Cys-loop receptors are allosterically regulated pentameric ligand-gated ion channels (pLGICs). In this work, we studied orphan receptor Alpo4 from an extreme thermophile worm Alvinella pompejana. Each Alpo4 subunit is composed of a β-sandwich extracellular domain (ECD) and a transmembrane domain (TMD) made of four trans-membrane α-helices M1-M4. In conclusion, Alpo4 has a pore structure consistent with a cation-selective channel, but with an unusually tight constriction at the 16’M position, the role of which remains unclear.

Given that Alpo4 shares a structural resemblance to the α4β2 nAChR and the 5-HT3R, we investigated whether acetylcholine or serotonin binds into the ligand-binding site. To this end, structures of Alpo4 purified in the absence of CHAPS and with an added, 1 mM acetylcholine or 1 mM serotonin were solved to a resolution of 3.9 Å and 6.2 Å, respectively (Figure 1—figure supplements 8 and 10). No density in the ligand-binding site was observed in the reconstructions. The cryo-EM reconstructions of Alpo4 obtained in the presence of acetylcholine and serotonin suggest that neither of the neurotransmitters binds Alpo4. This agrees with our electrophysiological experiments in various expression systems (Xenopus oocytes, HEK cells, lipid vesicles) indicating no agonist response to acetylcholine or serotonin (data not shown). The unmasked reconstruction (red) reaches 4.3 Å while the tight dynamic masked reconstruction (blue) reaches 3.9 Å.

>[5x]MAGSKVDKTLCRLGDITGLLIVLSVLVSRGLCQDCNNTNASSMADEKRLLKCILHDYDTAIRPVQNVSDVVNVALEVTVVKVIDLDEKEHVLTTNGWIYHEWNDFQLKWNPSDYSGLKKIRIPVDRIWTPDIVLFNNADESYRYVVDKLAVVYYTGKVMWVPHARLRSFCVLDLSRFPFDSQMCTLVFGSWTHDVSSVNVTLRNQSKVQYMIDGKEWQVTSVQPKRYQWTYNSNENYAGIITGIKLKRTSIYYQYVFIMPTVLLAFLTLLMPFIPPLGKERITYGIGLVLGCTLLLMMLSDRMPTELGNVPVVAAYLAYVFVMVAINLLFAIMAINMSMRDPKFGKVPGWVRWIFLTKLSKLVCLPVEPYTAVPADLAYEETAAARELLDMNNGTATADQRVSGSDTKPALDRTLEDIRRYLRLVATRTVVTPQLSHRDLVVQEWQQLTRVIDRLLFGSFLVLTVVITISMYAHY>AEGDDPAKAAFNSLQASATEYIGYAWAMVVVIVGATIGIKLFKKFTSKAS[25x];>MEQVADFDTIYQAMIQISVVLCFALGIIAGGQR[5x];>MSVLVYSFASFVLGWCLRSGITYFTRLME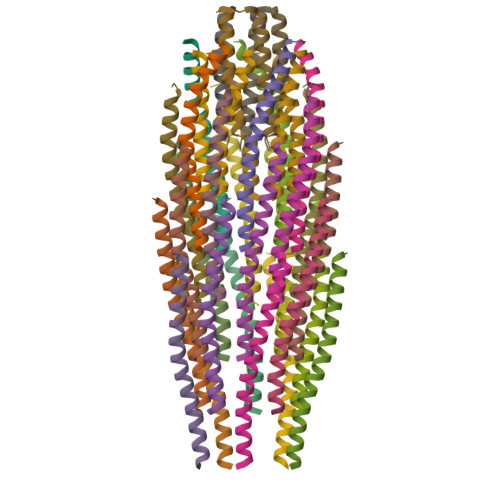TSS[5x]> LDPEEIRKRLEHTERQFRNRRKILIRGLPGDVTNQEVHDLLSDYELKYCFVDKYKGTAFVTLLNGEQAEAAINAFHQSRLRERELSVQLQPTDALLCVANLPPSLTQQQFEELVRPFGSLERCFLVYSERTGQSKGYGFAEYMKKDSAARAKSDLLGKPLGPRTLYVHWTDAGQLTPALLHSRCLCVDRLPPGFNDVDALCRALSAVHSPTFCQL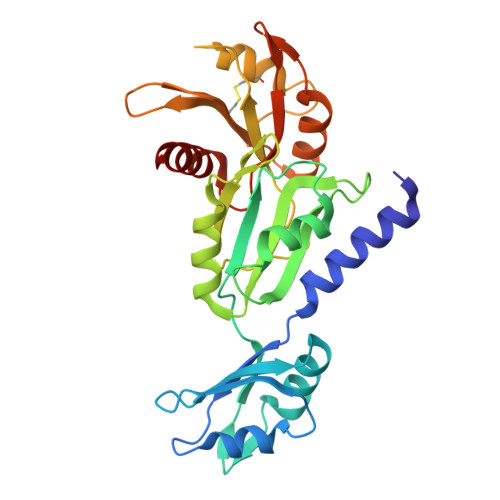ACGQDGQLKGFAVLEYETAEMAEEAQQQADGLSLGGSHLRVSFCAPGPPGRSMLAALIAAQATALNRG> SNAMVPTHHAGNGFAVASEQGRICALAARGQRDLRQCVRAYPSLFPNPPVDDTMLSALALSTAFIAPWCSAEQLRVANRASLWVTAEDWQVDRVATSDDAVRSIVSACQAVADGA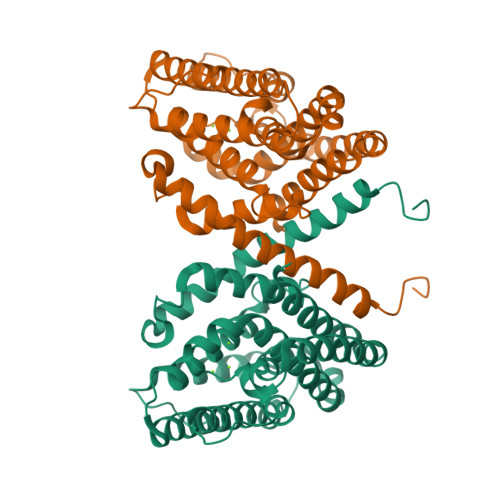APDVDCALGQLLAEIRDELATGAGFTEWQPVWREEVRRMLTADIREWEWRHSARPPSFAEYLDNADNYGASFVNVSHWIVTGDAQTRSHLPELIAASREVQRILRLSNDLASYERDIRSGDLNALLLVDREEVSRQLRDRIRACQDHLHALEVTCPREALYLAREAGFTTGFYHGADYWGDSER>[2x]MQVESLQNLQVKIRNDERNHSLTKKYLTDDIVKKYQATKTSLGGTLA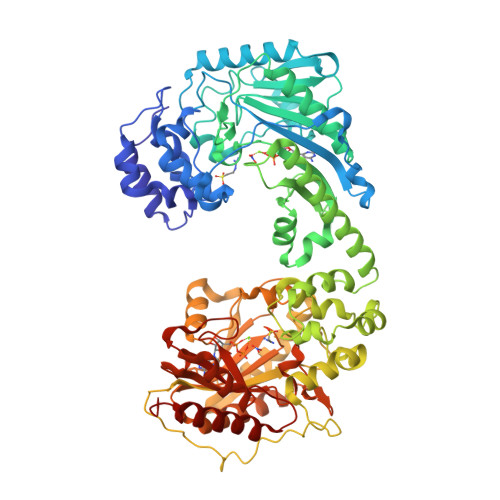QCVNTNAYNPGALLPRSCDLNAYETFRDFFDAVIADYHKVPDGKIQHPKSNFGDLKSLSFTDLNTYGNLVVSTRVRLGRTVEGFGFGPTLTKETRIELENKISTALHNLSGEYEGTYYPLTGMSEEDRIKLVNDHFLFRNDDNVLRDAGGYIDWPTGRGIFINKQKNFLVWINEEDHIRVISMQKGGGLTAVYKRLADAIQELSKSLKFAFNDRLGFITFCPSNLGTTLRASVHAKIPMLASLPNFKEICEKHGIQPRGTHGEHTESVGGIYDLSNKRRLGLTELDAVTEMHSGVRALLELEVMLQEYNKGAPEGVMPVEPLTYLAKLLEGASIEKCYTRKYLTPEIIKKYDGKRTTHGATLAHMIRNGAYNNRSICPRTGEAECYSTFIDYLDPLICDYHGVKDSAFKHPAPTFGDLSKLPFGDLDPTGKFIVSTRVRVGRSVEGFLFPTIMSKTDRIKLEQVISGALKGLTGEHAGTYYPLTDMKEEDRKQLVEDHFLFKNDDPVLRDAGGYRDWPVGRGIFHNNSKTFLVWVCEEDHMRIISMQQGGNLAAVYKRLIEGINAIGKSMKFAHSDKYGYITCCPSNLGTSMRASVLLKIPKLSSQPKKLDEICAKYMLQARGLYGEHTESPDGTYDISNKRRLGLTELQAAHEMAEGVAKMIEIEKGL Fpg/Nei DNA glycosylases are composed of two globular domains, an N-terminal domain rich in beta-structures and a C-terminal domain rich in alpha-structures. Most of them contain an original zinc finger (ZnF) motif (defining a new class of ZnF) comprising a β-hairpin structure with generally four cysteine residues coordinating the Zn2+ ion (type –C-X2(3)-C(H)-X16-18-C-X2-C-). Only the bacterial Fpg enzymes can excise 8-oxoG, the major oxidation product of purines. To further our understanding of the TXn mode of action, we solved several crystal structures of LlFpg bound to 14-mer [THF:C] (LRC) in the presence of thio-compounds.

The best inhibitor, TX13 (2-trifluoromethyl-6-thiopurine), is a monothio-compound; it was seven times more effective than 2TX, with an IC50appA of 7.5 µM. Using this method, we successfully resolved the structures of LRC with the moderately potent inhibitor 2TX (new crystal structure), high-efficiency inhibitors TX13, TX19, TX20, TX27, low-efficiency inhibitor TX15 and, TX19 in the presence of TCEP. In the absence of reducer and as previously observed with 2TX, all crystal structures showed that 2TX/TXn induced oxidation of the ZnF cysteine residues and the concomitant loss of the Zn2+ ion. With TXn, there was no clear electron density near the sulfur atoms of Cys248 and Cys268. Similar to the 2TX-containing crystal structure, the intramolecular disulfide bridge Cys245-S-S-Cys265 is also formed in the presence of TXn. A similar non-covalent binding at site II is also observed with TXn. The strictly conserved residues R260 of the ZnF loop and K57 of the β2-β3 loop of the N-terminal LlFpg domain are directly involved in the recognition of 2TX/TXn. The guanidinium group of the R260 side chain interacts with the unique sulfur atom of 2TX, TX15, TX20 and TX27, with the sulfur atom at the C8 position of TX19 (with or without TCEP) or with the N1 atom of the purine moiety of TX13. The epsilon amino group of the K57 side chain interacts with the sulfur atom of all 2TX/TXn compounds. Indeed, fine inspection of the crystal structures of C2 with that of the lesion recognition complex C1 resolved in the presence of 2TX, TX13, TX15, TX19, TX20 and TX27 showed that the 5′-overhanging cytosine of the damage-containing strand recognized by the second molecule (Mol-2) of LlFpg in C2 clashes with 2TX/TXn bound at the site II.

> PELPEVETVRRELEKRIVGQKIISIEATYPRMVLTGFEQLKKELTGKTIQGISRRGKYLIFEIGDDFRLISHLRMEGKYRLATLDAPREKHDHLTMKFADGQLIYADVRKFGTWELISTDQVLPYFLKKKIGPEPTYDEDFDEKLFREKLRKSTKKIKPYLLEQTLVAGLGNIYVDEVLWLAKIHPEKETNQLIESSIHLLHDSIIEILQKAIKLGGSSIRTYSALGSTGKMQNELQVYGKTGEKCSRCGAEIQKIKVAGRGTHFCPVCQQK> SLAKSAANKLDWAKVISSLRITGSTATQLSSFKKRNDEARRQLLELQSQPTEVDFSHYRSVLKNTSVIDKIESYVKQYKPVKIDASKQLQVIESFEKHAMTNAKETESLVSKELKDLQSTLDNIQSA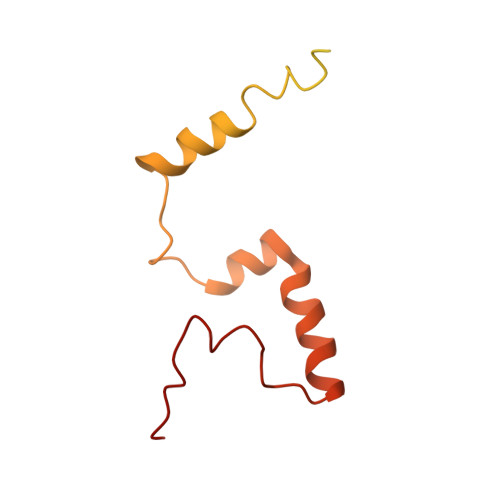RPFDELTVDDLTKIKPEIDAKVEEMVKKGKWDVPGYKDRFGNLNVM>HMNYRELIERARRTTAAEEYDISGRYPSVIAHAEGAWMTDLSGNRYVDLTGADAAVILGYRHPAVNEAITRQIRDYGTTFASTLSVPRVELAERMCERYECAEKVVFHKTGTEGTAMAVRLARAATGRELVLSSGYHGWHEWQMAGEEFGYQQSTGVVGFGYNEKALAKMLEAFGEQVAGVIVSPEVLYFDLDHYRRMSALCARYDVPFMLDEVYTGFRAGPKGVHGLGVPADVVVLGKGLANGHSLAAVMGRRDIIDAYDVSGIQGTYTREVPPMAAALAVFEVLDTPGVYEHAEAMGRRLADGMREILTGEGIPNWVGGPALMFDVVLPNDDLGWEIYKTAHDFGVYFEDSGTQ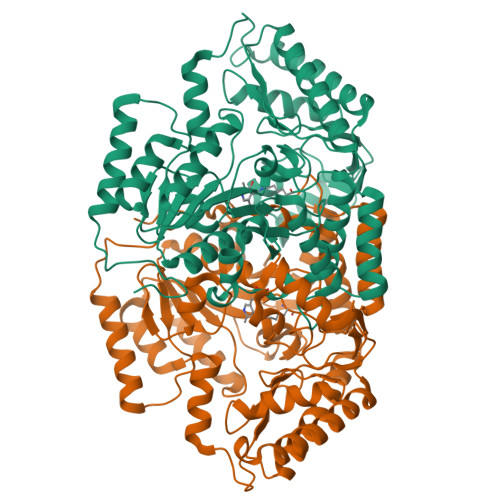LVTAAFDEAAVDHALTAFRKATRQVVADRPDIAPTSGGELTEERKLDFAEEAFGGLLRDDERTNALIDETIEKVVNRDRSIKPVLFPAQN[2x]> SNAMS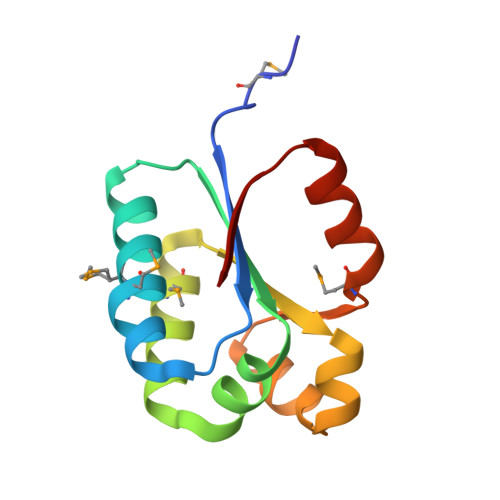ANDKLTILWTTDNKDTVFNMLAMYALNSKNRGWWKHINIILWGASVKLVANDTQVQTEILEMLQSGITIEACQDCCENFGVASIITNLGITVRYMGIPLTEYLKNGEKILSI> GEFKPSACRNLFGPVDHEELTRDLEKHCRDMEEASQRKWNFDFQNHKPLEGKYEWQEVEKGSLPEFYYRPPKGACKVPAQ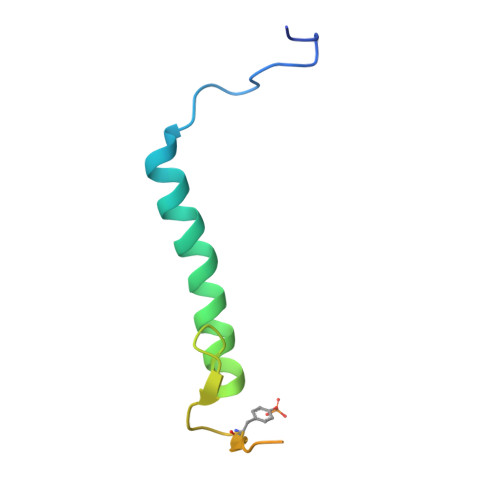ES> SKPTVQGKIGECKLRGQGRMANFDGMDMSHKMALSSTNEIETNEGLAGTSLDVMDLSRVLSIPNYWDRFTWKTSDVINTVLWDNYVSPFKVKPYSATITDRFRCTHMGKV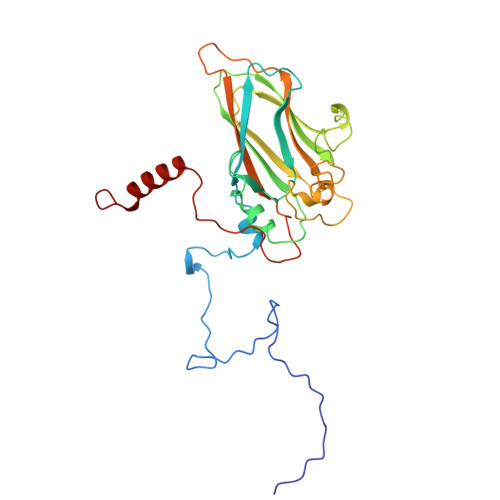ANAFTYWRGSMVYTFKFVKTQYHSGRLRISFIPYYYNTTISTGTPDVSRTQKIVVDLRTSTAVSFTVPYIGSRPWLYCIRPESSWLSKDNTDGALMYNCVSGIVRVEVLNQLVAAQNVFSEIDVICEVNGGPDLEFAGPTCPRYVPYAGDFTLADTRKIEAERTQEYSNNED>MAKAHIELTINGHPVEALVEPRTLLIHFIREQQ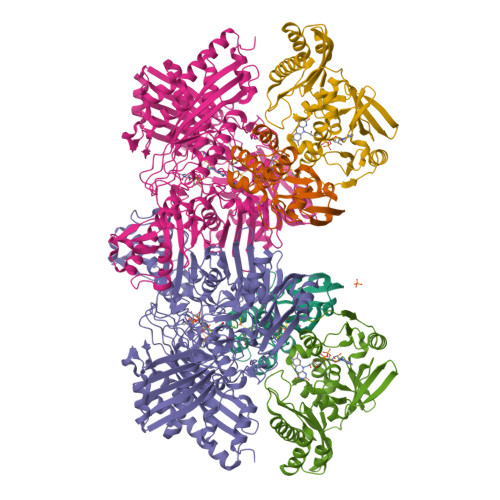NLTGAHIGCDTSHCGACTVDLDGMSVKSCTMFAVQANGASITTIEGMAAPDGTLSALQEGFRMMHGLQCGYCTPGMIMRSHRLLQENPSPTEAEIRFGIGGNLCRCTGYQNIVKAIQYAAAKINGVPFEEAAE[2x];>[2x]MNIQTTVEPTSAERAEKLQGMGCKRKRVEDIRFTQGKGNYVDDVKLPGMLFGDFVRSSHAHARIKSIDTSKAKALPGVFAVLTAADLKPLNLHYMPTLAGDVQAVLADEKVLFQNQEVAFVVAKDRYVAADAIELVEVDYEPLPVLVDPFKAMEPDAPLLREDIKDKMTGAHGARKHHNHIFRWEIGDKEGTDATFAKAEVVSKDMFTYHRVHPSPLETCQCVASMDKIKGELTLWGTFQAPHVIRTVVSLISGLPEHKIHVIAPDIGGGFGNKVGAYSGYVCAVVASIVLGVPVKWVEDRMENLSTTSFARDYHMTTELAATKDGKILAMRCHVLADHGAFDACADPSKWPAGFMNICTGSYDMPVAHLAVDGVYTNKASGGVAYRCSFRVTEAVYAIERAIETLAQRLEMDSADLRIKNFIQPEQFPYMAPLGWEYDSGNYPLAMKKAMDTVGYHQLRAEQKAKQEAFKRGETREIMGIGISFFTEIVGAGPSKNCDILGVSMFDSAEIRIHPTGSVIARMGTKSQGQGHETTYAQIIATELGIPADDIMIEEGNTDTAPYGLGTYGSRSTPTAGAATAVAARKIKAKAQMIAAHMLEVHEGDLEWDVDRFRVKGLPEKFKTMKELAWASYNSPPPNLEPGLEAVNYYDPPNMTYPFGAYFCIMDIDVDTGVAKTRRFYALDDCGTRINPMIIEGQVHGGLTEAFAVAMGQEIRYDEQGNVLGASFMDFFLPTAVETPKWETDYTVTPSPHHPIGAKGVGESPHVGGVPCFSNAVNDAYAFLNAGHIQMPHDAWRLWKVGEQLGLHV;>[2x]MIPGSFDYHRPKSIADAVALLTKLGEDARPLAGGHSLIPIMKTRLATPEHLVDLRDIGDLVGIREEGTDVVIGAMTTQHALIGSDFLAAKLPIIRETSLLIADPQIRYMGTIGGNAANGDPGNDMPALMQCLGAAYELTGPEGARIVAARDYYQGAYFTAIEPGELLTAIRIPVPPTGHGYAYEKLKRKIGDYATAAAAVVLTMSGGKCVTASIGLTNVANTPLWAEEAGKVLVGTALDKPALDKAVALAEAITAPASDGRGPAEYRTKMAGVMLRRAVERAKARAKN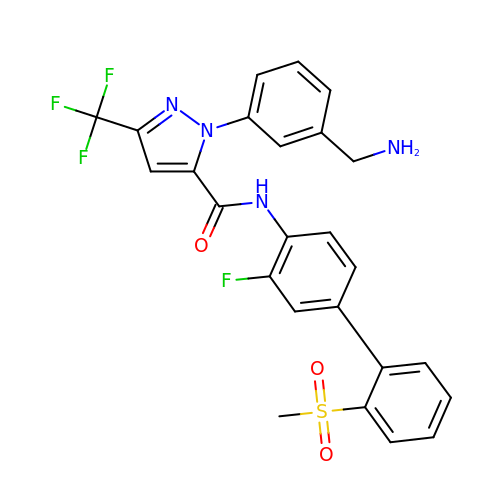1-[3-(aminomethyl)phenyl]-N-[3-fluoro-2'-(methylsulfonyl)biphenyl-4-yl]-3-(trifluoromethyl)-1H-pyrazole-5-carboxamide | C25 H20 F4 N4 O3 S | ZLUOAFAJSUPHOG-UHFFFAOYSA-N> HSLKPWNTFGIDHNAQHIVCAEDEQQLLNAWQYATAEGQPVLILGEGSNVLFLEDYRGTVIINRIKGIEIHDEPDAWYLHVGAGENWHRLVKYTLQEGMPGLENLALIPGCVGSSPIQNIGAYGVELQRVCAYVDSVELATGKQVRLTAKECRFGYRDSIFKHEYQDRFAIVAVGLRLPKEWQPVLTYGDLTR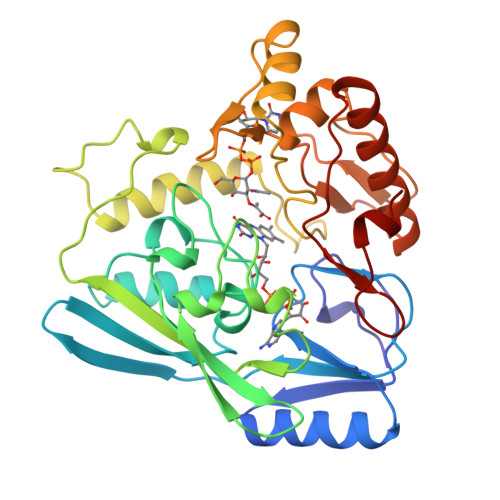LDPTTVTPQQVFNAVCHMRTTKLPDPKVNGNAGSFFKNPVVSAETAKALLSQFPTAPNYPQADGSVKLAAGWLIDQCQLKGMQIGGAAVHRQQALVLINEDNAKSEDVVQLAHHVRQKVGEKFNVWLEPEVRFIGASGEVSAVETIS>[4x]MSLRIAIVGAGALGLYYGALLQRSGEDVHFLLRRDYEAIAGNGLKVFSINGDFTLPHVKGYRAPEEIGPMDLVLVGLKTFANSRYEELIRPLVEEGTQILTLQNGLGNEEALATLFGAERIIGGVAFLCSNRGEPGEVHHLGAGRIILGEFLPRDTGRIEELAAMFRQAGVDCRTTDDLKRARWEKLVWNIPFNGL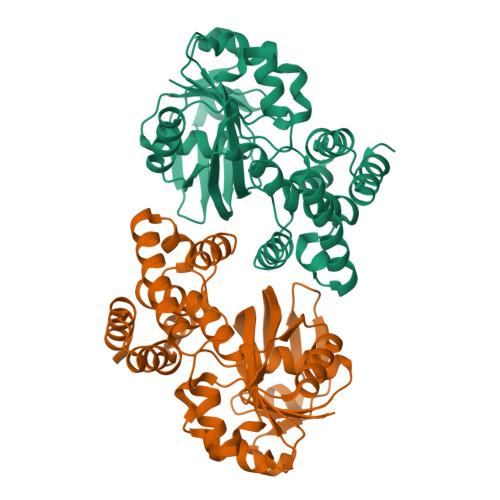CALLQQPVNLILARDVSRKLVRGIMLEVIAGANAQGLATFIADGYVDDMLEFTDAMGEYKPSMEIDREEGRPLEIAAIFRTPLAYGAREGIAMPRVEMLATLLEQATGEGHHHHHH> MADLDPSQYFETRSRQIQELRKTHEPNPYPHKFHVSISNPEFLAKYAHLKKGETLPEEKVSIAGRIHAKRESGSKLKFYVLHGDGVEVQLMSQLQDYCDPDSYEKDHDLLKRGDIVGVEGYVGRTQPKKGGEGEVSVFVSRVQLLTPCLHMLPADHFGFKDQETRYRKRYLDLIMNKDARNRFITRSEIIRYIRRFLDQRKFIEVETPMMNVIAGGATAKPFITHHNDLDMDMYMRIAPELFLKQLVVGGLDRVYEIGRQFRNEGIDMTHNPEFTTCEFYQAYADVYD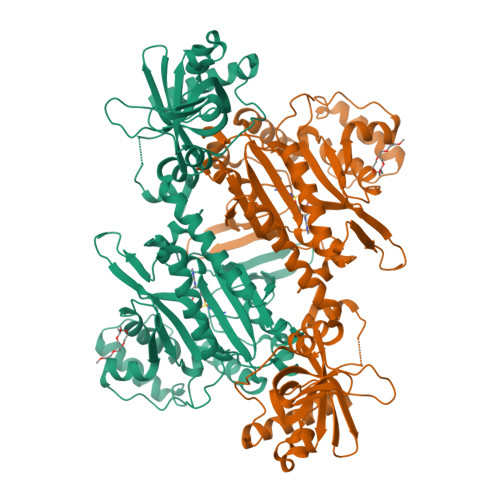LMDMTELMFSEMVKEITGSYIIKYHPDPADPAKELELNFSRPWKRINMIEELEKVFNVKFPSGDQLHTAETGEFLKKILVDNKLECPPPLTNARMLDKLVGELEDTCINPTFIFGHPQMMSPLAKYSRDQPGLCERFEVFVATKEICNAYTELNDPFDQRARFEEQARQKDQGDDEAQLVDETFCNALEYGLPPTGGWGCGIDRLAMFLTDSNTIREVLLFPTLKPDVLEHHHHHH> DAPESWDWSKKGVITKVKFQGQCGSGWAFSATGAIEAAHAIATGNLVSLSEQELIDCVDESEGCYNGWHYQSFEWVVKHGGIASEADYPYKARDGKCKANEIQDKVTIDNYGVQILSNESTESEAESSLQSFVLEQPISVSIDAKDFHFYSGGIYDGGNCSSPYGINHFVLIVGYGSEDGVDYWIAKNSWGEDWGIDGYIRIQRNTGNLLGVCGMNYFASYPIIEKSETLK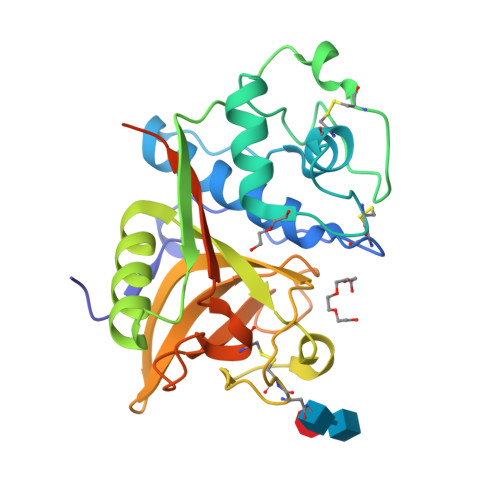FGRVKADPRVEHSPL>[54x]MNNLYRDLAPVTEAA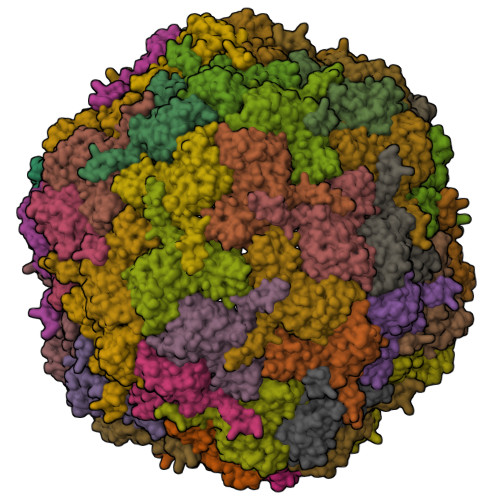WAEIELEAARTFKRHIAGRRVVDVSDPGGPVTAAVSTGRLIDVKAPTNGVIAHLRASKPLVRLRVPFTLSRNEIDDVERGSKDSDWEPVKEAAKKLAFVEDRTIFEGYSAASIEGIRSASSNPALTLPEDPREIPDVISQALSELRLAGVDGPYSVLLSADVYTKVSETSDHGYPIREHLNRLVDGDIIWAPAIDGAFVLTTRGGDFDLQLGTDVAIGYASHDTDTVRLYLQETLTFLCYTAEASVALSH> MTATVLLEVPFSARGDRIPDAVAELRTREPIRKVRTITGAEAWLVSSYALCTQVLEDRRFSMKETAAAGAPRLNALTVPPEVVNNMGNIADAGLRKAVMKAITPKAPGLEQFLRDTANSLLDNLITEGAPADLRNDFADPLATALHCKVLGIPQEDGPKLFRSLSIAFMSSADPIPAAKINWDRDI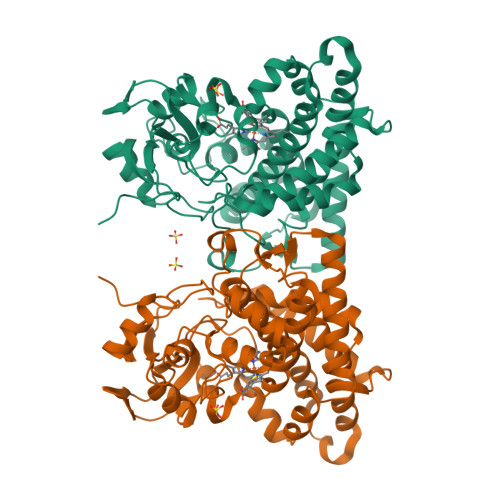EYMAGILENPNITTGLMGELSRLRKDPAYSHVSDELFATIGVTFFGAGVISTGSFLTTALISLIQRPQLRNLLHEKPELIPAGVEELLRINLSFADGLPRLATADIQVGDVLVRKGELVLVLLEGANFDPEHFPNPGSIELDRPNPTSHLAFGRGQHFCLGSALGRRHAQIGIEALLKKMPGVDLAVPIDQLVWRTRFQRRIPERLPVLW> TGRPEWIWLALGTALMGLGTLYFLVKGMGVSDPDAKKFYAITTLVPAIAFTMYLSMLLGYGLTMVPFGGEQNPIYWARYADWLFTTPLLLLDLALLVDADQGTILALVGADGIMIGTGLVGALTKVYSYRFVWWAISTAAMLYILYVLFFGFTSKAESMRPEVASTFKVLRNVTVVLWSAYPVVWLIGSEGAGIVPLNIETLLFMVLDVSAKVGFGLILL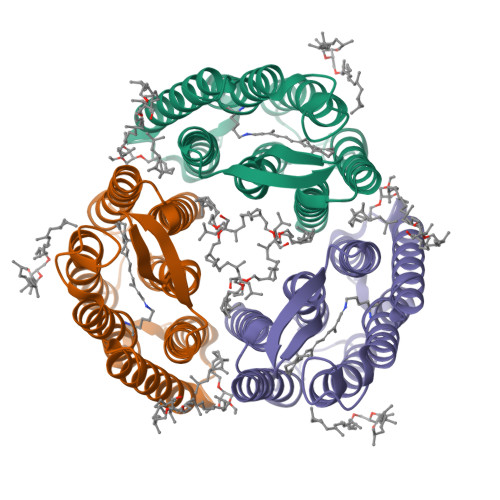RSRAIFGE> MSHHHHHHSMSAAPDSPSSALAALPKDVPNSQPEMVEAVKKHILNMLHLKKRPDVTQPVPKAALLNAIRKLHVGKVGENGYVEIEDDIGRRAEMNELMEQTSEIITFAESGTARKTLHFEISKEGSDLSVVERAEVWLFLKVPKANRTRTKVTIRLFQQQKHPQGSLDTGEEAEEVGLKGERSELLLSEKVVDARKSTWHVFPVSSSIQRLLDQGKSSLDVRIACEQCQESGASLVLLGEEKEQSHRPFLMLQARQSEDHPHRRRRRGLECDGKVNICCKKQFFVSFKDIGWNDWIIAPSGYHANYCEGECPSHIAGTSGSSLSFHSTV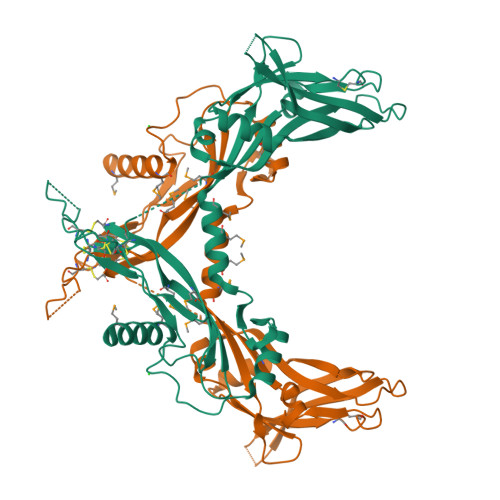INHYRMRGHSPFANLKSCCVPTKLRPMSMLYYDDGQNIIKKDIQNMIVEECGCS>[2x]MGHHHHHHFDHSFSFDCQDKVILVVEDDYDIGDIIENYLKREGMSVIRAMN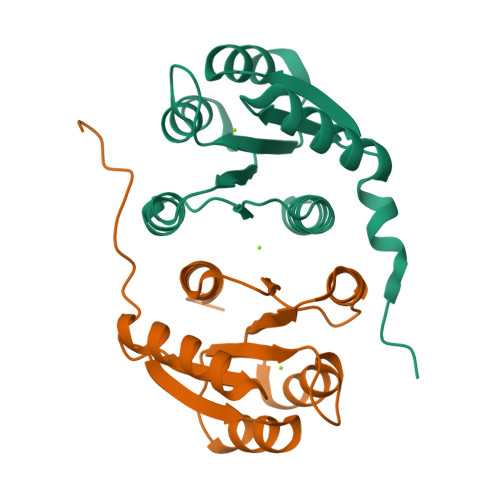GKQAIELHASQPIDLILLDIKLPELNGWEVLNKIRQKAQTPVIMLTALDQDIDKVMALRIGADDFVVAPFNPNEVIARVQAVLRRTQFANKAT>[2x]MLDNSFYTAEVQGPYETASIGRLELEEGGVIEDCWLAYATAGTLNEDKSNAILIPTWYSGTHQTWFQQYIGTDHALDPSKYFIISINQIGNGLSVSPANTA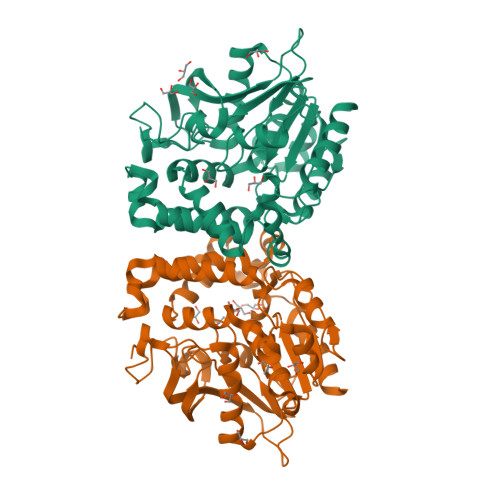DDSISMSKFPNVRIGDDVVAQDRLLRQEFGITELFAVVGGSMGAQQTYEWIVRFPDQVHRAAPIAGTAKNTPHDFIFTQTLNETVEADPGFNGGEYSSHEEVADGLRRQSHLWAAMGFSTEFWKQEAWRRLGLESKESVLADFLDPLFMSMDPNTLLNNAWKWQHGDVSRHTGGDLAAALGRVKAKTFVMPISEDMFFPVRDCAAEQALIPGSELRVIEDIAGHLGLFNVSENYIPQIDKNLKELFES[[[(2R,3R,4S,5R)-3,4-bis(oxidanyl)-5-(phosphonooxymethyl)oxolan-2-yl]oxy-oxidanyl-phosphoryl]amino]phosphonic acid | C5 H14 N O13 P3 | 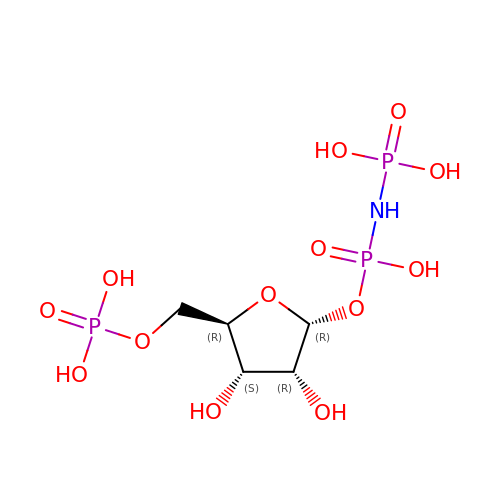FCRMTSGXHCKCEX-TXICZTDVSA-N>[2x]XGEIAQQLKEIAKQLKEIAW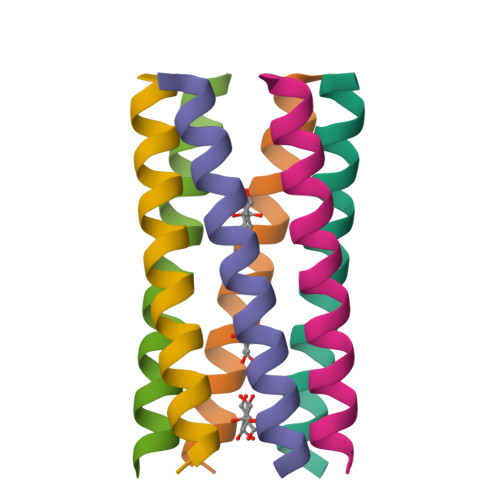QLKEIAQQLKGX> NDPIANAVESAVSALADTTISRVTAANTTASTHSLGTGRVPALQAAETGASSNASDENLVETRCVMNRNGVNEASVEHFYSRAGLVGVVEVKDSGTSLDGYTVWPIDVMGFVQQRRKLELSTYMRFDAEFTFVSNLSNSTTPGMLLQYMYVPPGAPKPDGRKSYQWQTATNPSVFAKLSDPPPQVSVPFMSPATAYQWFYDGYPTFGEHKQATNLQYGQCPNNMMGHFAIRTVSESTTGKNVHVRVYMRIKHVRAWVPRPLRSQAYMVKNYPTYSQTITNTATDRASITTTDYEGGVPASPQRTS;> MGAQVSTQKSGSHETRNVATEGSTINFTNINYYKDSYAASASRQDFAQDPAKF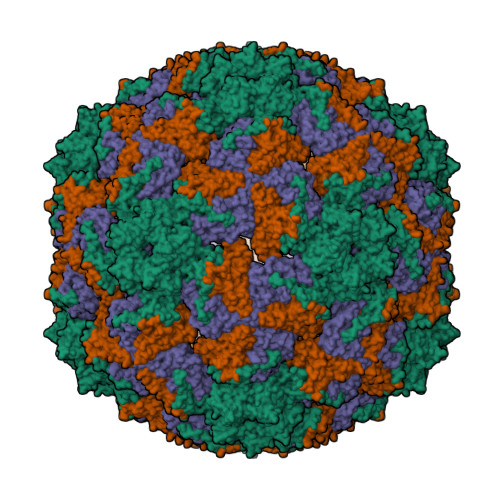TRPVLDTIREVAAPLQSPSVEACGYSDRVAQLTVGNSTITTQEAANIVLSYGEWPEYCPSTDATAVDKPTRPDVSVNRFYTLSTKSWKTESTGWYWKFPDVLNDTGVFGQNAQFHYLYRSGFCMHVQCNASKFHQGALLVAAIPEFVIAASSPATKPNGRGLYPDFAHTNPGKDGQEFRDPYVLDAGIPLSQALVFPHQWINLRTNNCATIIMPYVNALPFDSALNHSNFGLVVIPISPLKYCNGATTEVPVTLTIAPLNSEFSGLRQAIKQ;> GFPTELKPGTNQFLTTDDGTSPPILPGFEPTPLIHIPGEFTSLLDLCQIETILEVNNTTGTIGVSRLLIPVRAQNNVDQLCASFQVDPGRNGPWQSTMVGQICRYYTQWSGSLKVTFMFTGSFMATGKMLIAYTPPGSAQPATREAAMLGTHIVWDFGLQSSVTLVIPWISNTHFRAVKIGGVYDYYATGIVTIWYQTNFVVPPDTPTEANIIALGAAQKNFTLKLCKDTDEIQQTAAYQ>[2x]MSAYNSKVKKAVIPVAGLGTRMLPATKAIPKEMLPLVDKPLIQ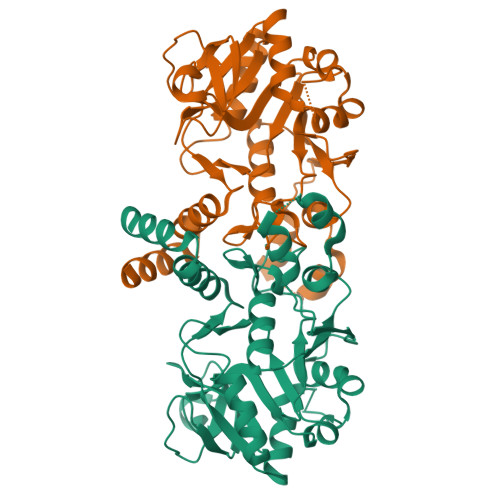YVVNECIAAGINEIVLVTHSSKNSIENHFDTSFELEAMLEKRVKRQLLEEIQSICPPHVTIMQVRQGLAKGLGHAVMCAWPVIGNEPVAVILPDVILDEYESDLSKDNLAEMIRRFDETGHSQIMVEPVADVTAYGVVDCQGAQLNPGDSAPMVGVVEKPKADQAPSNLAVVGRYVLSADIWPLLAKTPPGAGDEIQLTDSIAMLMEKETVEAYHLKGVSHDCGNKLGYMQAFVEYGVRHETLGSDFKAWLESAVGNKK> MGPSFNPVRFLELPIDIRKEVYFHLDGNFCGAHPYPIDILYKSNDVELPGKPSYKRSKRSKKLLRYMYPVFATYLNIFEYSPQLIEKWLEYAFWLRYDCLVLDCFKVNHLYDGTLIDALEWTYLDNELRLAYFNKASMLEVWYTFKEYKKWVIDSVAFDELDLLNVSNIQFNIDNLTPQLVDKCLSILEQKDLFATIGEVQFGQDEEVGEEKDVDVSGANSDENSSPSSTIKNKKRSASKRSHSDNGNVGATHNQLTSISVIRTIRSMESMKSLRKITVRGEKLYELLINFHGFRDNPGK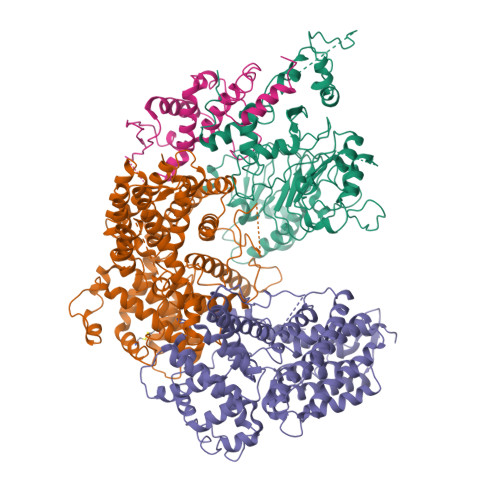TISYIVKRRINEIRLSRMNQISRTGLADFTRWDNLQKLVLSRVAYIDLNSIVFPKNFKSLTMKRVSKIKWWNIEENILKELKVDKRTFKSLYIKEDDSKFTKFFNLRHTRIKELDKSEINQITYLRCQAIVWLSFRTLNHIKLQNVSEVFNNIIVPRALFDSKRVEIYRCEKISQVLVIGSRSGSENLYFQGSKRRWKKNFIAVSAANRFKKISSSGAL;>[2x]MFNRTTQLKSKHPCSVCTRRKVKCDRMIPCGNCRKRGQDSECMKSTKLITASSSKEYLPDLLLFWQNYEYWITNIGLYKTKQRDLTRTPANLDTDTEECMFWMNYLQKDQSFQLMNFAMENLGALYFGSIGDISELYLRVEQYWDRRADKNHSVDGKYWDALIWSVFTMCIYYMPVEKLAEIFSVYPLHEYLGSNKRLNWEDGMQLVMCQNFARCSLFQLKQCDFMAHPDIRLVQAYLILATTTFPYDEPLLANSLLTQCIHTFKNFHVDDFRPLLNDDPVESIAKVTLGRIFYRLCGCDYLQSGPRKPIALHTEVSSLLQHAAYLQDLPNVDVYREENSTEVLYWKIISLDRDLDQYLNKSSKPPLKTLDAIRRELDIFQYKVDSLEEDFRSNNSRFQKFIALFQISTVSWKLFKMYLIYYDTADSLLKVIHYSKVIISLIVNNFHAKSEFFNRHPMVMQTITRVVSFISFYQIFVESAAVKQLLVDLTELTANLPTIFGSKLDKLVYLTERLSKLKLLWDKVQLLDSGDSFYHPVFKILQNDIKIIELKNDEMFSLIKGLGSLVPLNKLRQESLLEEEDENNTEPSDFRTIVEEFQSEYNISDILSGSGGSGENLYFQ;> MVTSNVVLVSGEGERFTVDKKIAERSLLLKNYLNDMHDSNLQNNSDSESDSDSETNHKSKDNNNGDDDDEDDDEIVMPVPNVRSSVLQKVIEWAEHHRDSNFPDEDDDDSRKSAPVDSWDREFLKVDQEMLYEIILAANYLNIKPLLDAGCKVVAEMIRGRSPEEIRRTFNIVNDFTPEEEAAIRRENEWAEDR>[6x]MKTGADRFLEELPEVAESFKNFREAVRSEGKLTEREKLLISVACSVAVRCDACTRRHA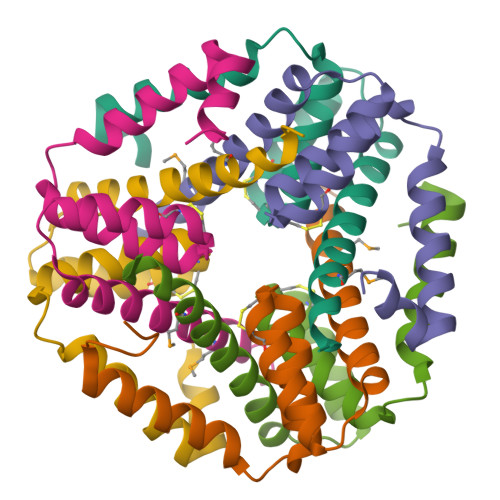EEALEAGITEGELAEAAAVAALIRAGSAMNTASAIFRD> GPLGSEEGLFSQKSFLVLGFSNENESNIANIIKENAGK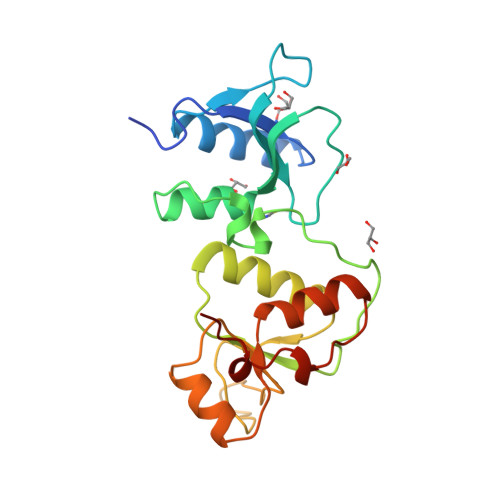IMSLLSRTVADYAVVPLLGCEVEATVGEVVTNTWLVTCIDYQTLFDPKSNPLFTPVPVMTGMTPLEDCVISFSQCAGAEKESLTFLANLLGASVQEYFVRKSNAKKGMFASTHLILKERGGSKYEAAKKWNLPAVTIAWLLETARTGKRADESHFLIENSTKEER> MVLKQRANYLGFLIVFFTAFLVEAVPIKRQSNSTVDSLPPLIPSRTSAPSSSPSTTDPEAPAMSRNGPLPSDVETKYGMALNATSYPDSVVQAMDGGIRAATSQEINELTYYTTLSANSYCRTVIPGATWDCIHCDATEDLKIIKTWSTLIYDTNAMVARGDSEKTIYIVFRGSSSIRNWIADLTFVPVSYPPVSGTKVHKGFLDSYGEVQNELVATVLDQFKQYPSYKVAVTGHSLGGATALLCALDLYQREEGLSSSNLFLYTQGQPRVGDPAFANYVVSTGIPYRRTVNERDIVPHLPPAAFGFLHAGEEYWITDNSPETVQVCTSDLET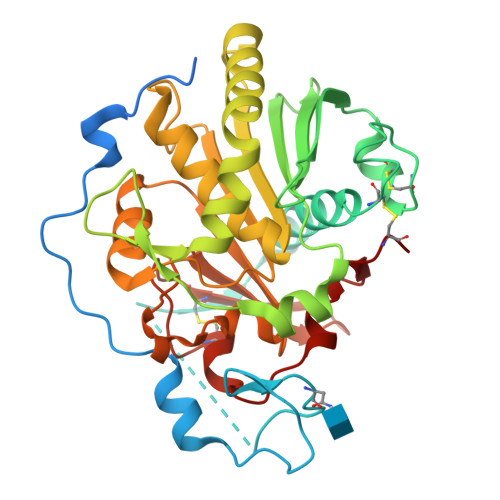SDCSNSIVPFTSVLDHLSYFGINTGLCT N-[(2,3-dihydroxyphenyl)carbonyl]-O-[(2S)-2-{[(2,3-dihydroxyphenyl)carbonyl]amino}-3-(L-seryloxy)propanoyl]-L-serine 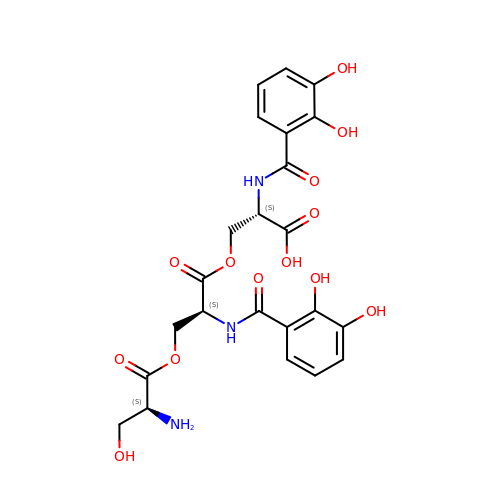| C23 H25 N3 O13 | AVZOYWMPRGKOPV-IHRRRGAJSA-N> MSHHHHHHSLGNKLSITDVKAIQGKKVLVRVDFNVPIENGVIKDTNRITATLPTIHHLKKEGAAKIILISHCGRPDGTKNLKYTLKPVAETLGTLLGEEVLFLSDCVGEEVAAQINQAKDNSVILLENLRFHVEEEGKGVDAAGNKIKASKEDMEKFQNELTKLGDVFINDAFGTAHRAHSSMVGIKMNVKASGFLMKKELEYFSKALENPQRPLLAILGGAKVSDKIQLIKNLLDKVDKMIIGGGMAYTFKYVLN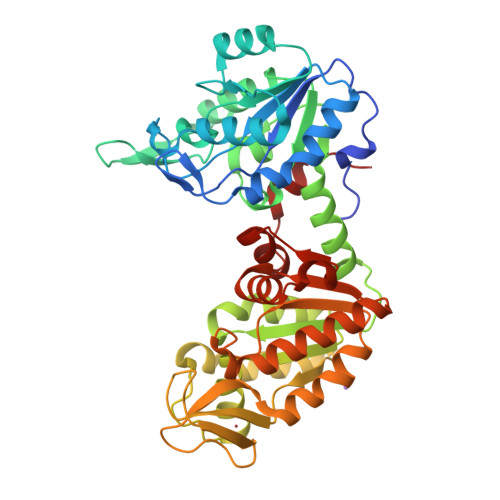NMKIGDSLFDEAGSKIVNEIMEKAKAKNVEIYLPVDFKVADKFDNNANTKVVTDEEGIEDKWMGLDAGPKSIENYKDVILSSKTIIWNGPQGVFEMPNFAKGSIECLNLVIEATKKGAISIVGGGDTASLVEQQQKKNEISHVSTGGGASLELLEGKELPGVVALSSK> MAGAIIENMSTKKLCIVGGILLVFQIIAFLVGGLIAPGPTTAVSYMSVKCVDARKNHHKTKWFVPWGPNHCDKIRDIEEAIPREIEANDIVFSVHIPLPHMEMSPWFQFMLFILQLDIAFKLNNQIRENAEVSMDVSLAYRDDAFAEWTEMA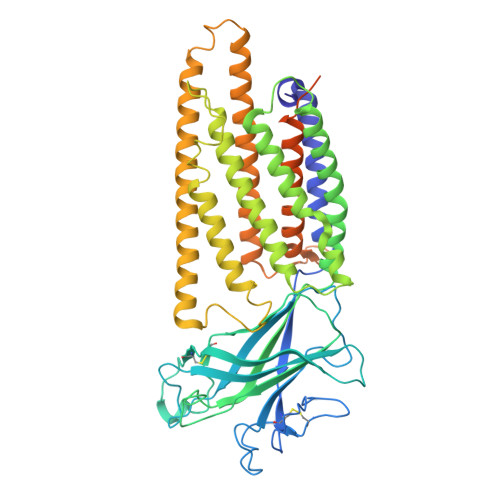HERVPRKLKCTFTSPKTPEHEGRYYECDVLPFMEIGSVAHKFYLLNIRLPVNEKKKINVGIGEIKDIRLVGIHQNGGFTKVWFAMKTFLTPSIFIIMVWYWRRITMMSRPPVLLEKVIFALGISMTFINIPVEWFSIGFDWTWMLLFGDIRQGIFYAMLLSFWIIFCGEHMMDQHERNHIAGYWKQVGPIAVGSFCLFIFDMCERGVQLTNPFYSIWTTDIGTELAMAFIIVAGICLCLYFLFLCFMVFQVFRNISGKQSSLPAMSKVRRLHYEGLIFRFKFLMLITLACAAMTVIFFIVSQVTEGHWKWGGVTVQVNSAFFTGIYGMWNLYVFALMFLYAPSHKNYGEDQSNGDLGVHSGEELQLTTTITHVDGPTEIYKLTRKEAQEAENLYFQSHHHHHHHHHHDYKDDDDK>[2x]SNAMTTDKQTSINLALSTINGKWKLSLMDELFQGTKRNGELMRALDGITQRVLT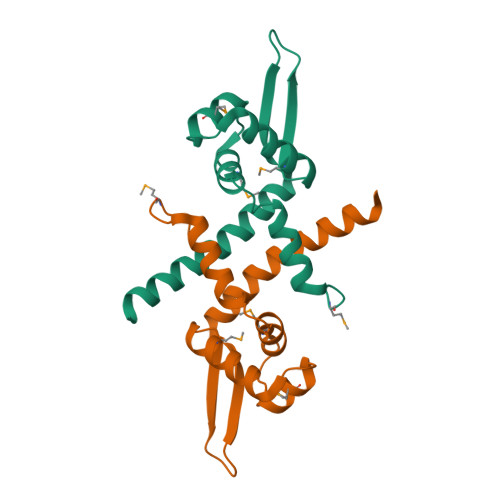DRLREMEKDGLVHRESFNELPPRVEYTLTPEGYALYDALSSLCHWGETFAQKKARLNK2-amino-7-(propan-2-yl)-3-(1H-tetrazol-5-yl)-5H-[1]benzopyrano[2,3-b]pyridin-5-one | C16 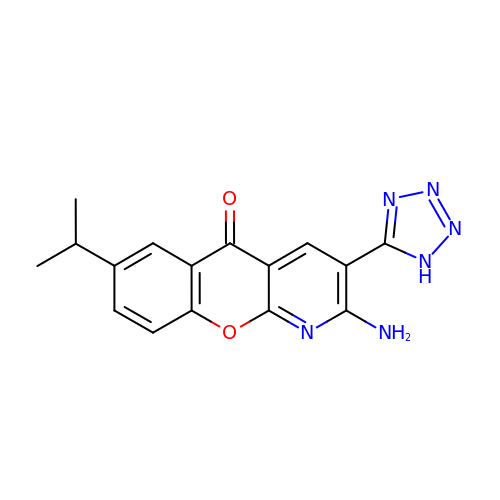H14 N6 O2 | YHCFWEQYIPEHCK-UHFFFAOYSA-N>CTGIRYSDGSGNLYLARNLDWTSDFGERVVVTPTGYTTKSPFGAVPAIRHAVIGMGIVQEDTPLYFDCGNDAGLAVAGLNFPGYAQYATEAVDGATNVAAFEFPLWVASQFASVDEVEAALADVVIVDRPINDKYPSSLLHWIIGDSKRAIVVEYTSDGLHVFDDDVDVLANQPGFGWHHENLRNYLNASPDFPEKIVLNRADLVPFGSGSLMRGIPGDYYSPSRFVRAAYVHAHYPGKSTEEENVSRAFHTLQQVAMVDGSAAMGSGEFEKTTYTGLFSSRTMTYYWNTYEDPAVRSVAMADHAADGTELVVVLEHHHHHH[2x]

Bile salt hydrolases (BSHs) catalyze the amino acid deconjugation reactions required to liberate free bile acids for subsequent and successive modifications and metabolism. The BSHs belong to the N-terminal nucleophile hydrolase (Ntn-hydrolase) superfamily, which is characterized by an αββα core structure that is subject to autoactivation. Here, we identify and describe the BSH from a common member of the Plains bison microbiome, Arthrobacter citreus (BSHAc). Steady-state kinetic analyses demonstrated that BSHAc is a broad-spectrum hydrolase with a preference for glycine-conjugates and deoxycholic acid (DCA).

To better understand the interactions between BSHAc and AAA-10, we crystallized the enzyme after soaking it with the inhibitor for 18 h in 0.1 M MES, pH 6.0 at room temperature. X-ray diffraction data were collected that resulted in the refinement of 1.6 Å resolution model showing a covalent adduct. Structural characterization of BSHAc reacted with AAA-10 showed covalent modification of the N-terminal cysteine nucleophile, providing molecular details for an enzyme-stabilized product formed from this mechanism-based inhibitor’s α-fluoromethyl ketone warhead. The inhibitor was modeled at full occupancy with the BSH oxyanion hole accommodating the product’s ketone oxygen atom. C12 of the LCA-based AAA-10 was notably solvent-exposed and a series of polar and non-polar interactions appear to stabilize the inhibitor structure. Specifically, Trp22, Phe26, and the nearby Tyr136 shift to accommodate the inhibitor, enclosing it from solvent. Finally, two of the C3-sulfate oxygens interact with the backbone amides of Ile132 and Ser139, and a series of water molecules are also present in the inhibitor-occupied active site. The position of the atoms in the SB loop differs significantly between unbound and AAA-10 bound BSHAc models. While the apparent flexibility of this loop allows for the C3-SO4 group of AAA-10 to bind, there is clear displacement of residues that are likely to have roles in stabilizing a substrate. Accordingly, this SB loop of BSHAc may impede rather than accommodate inhibitor binding.>[2x]MNGAIKVGAWGGNGGS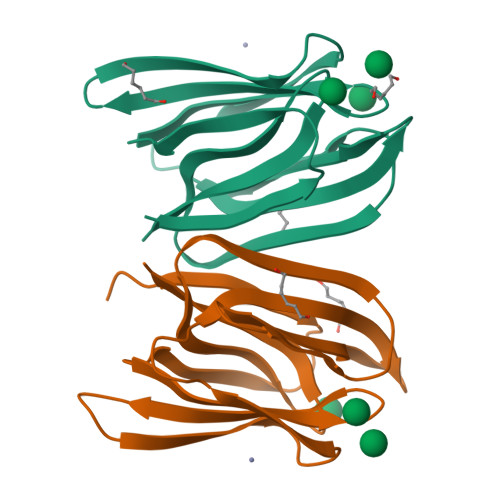AFDMGPAYRIISVKIFSGDVVDAVDVTFTYYGKTETRHFGGSGGTPHEIVLQEGEYLVGMKGEFGNYHGVVVVGKLGFSTNKKSYGPFGNTGGTPFSLPIAAGKISGFFGRGGDFIDAIGVYLEP>MKKPRIDMHSHFFPRISEQEAAKFDANHAPWLQVSAKGDTGSIMMGKNNFRPVYQALWDPAFRIEEMDAQGVDVQVTCATPVMFGYTWEANKAAQWAERMNDFALEFAAHNPQRIKVLAQVPLQDLDLACKEASRAVAAGHLGIQIGNHLGDKDLDDATLEAFLTHCANEDIPILVHPWDMMGGQRMKKWMLPWLVAMPAETQLAILSLILSGAFERIPKSLKICFGHGGGSFAFLLGRVDNAWRHRDIVREDCPRPPSEYVDRFFVDSAVFNPGALELLVSVMGEDRVMLGSDYPFPLGEQKIGGLV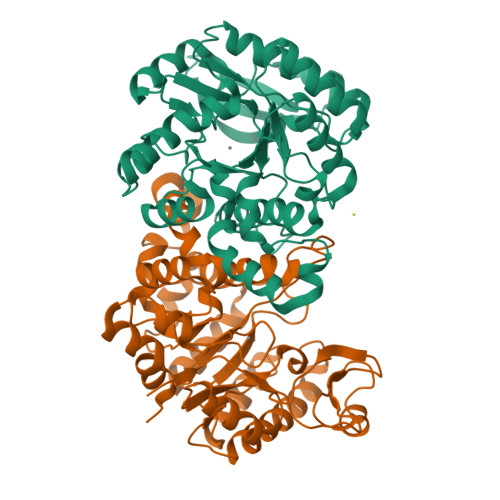LSSNLGESAKDKIISGNASKFFNINV[2x]>[2x]GGRMQLTADQVEKYKSDGYVLLEGAFSPEEVHVMRQALKKDQEVQGPHRILEEDGRTVRALYASHTRQSVFDQLSRSDRLLGPATQLLECDLYIHQFKINTKRAFGGDSWAWHQDFIVWRDTDGLPAPRAVNVGVFLSDVTEFNGPVVFLSGSHQR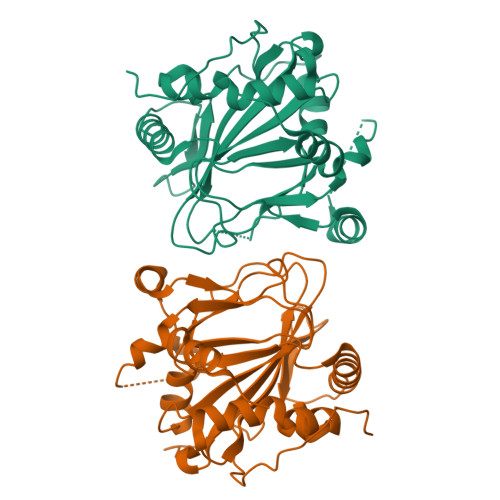GTVERKARETSRSDQHVDPDDYSMTPAELSQMVEKHPMVSPKAASGSVMLFHPEIIHGSAPNISPFARDLLIITYNDVANAPKPAGEPRPEYVIGRDTTPLVSRSGPLHEAA>AEGDDPAKAAFDSLQASATEMIGYAWAMVVVIVGATIG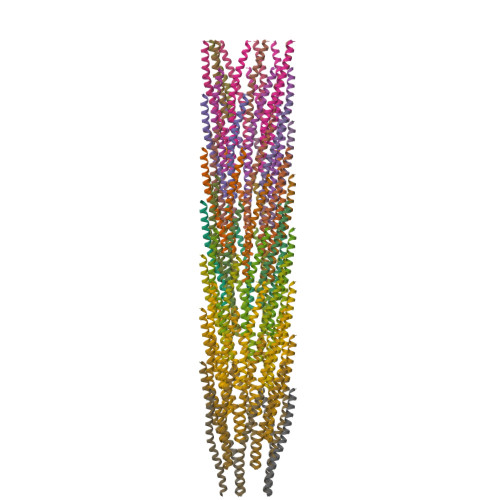IKLFKKFTSKAS[75x]>[2x]MAHHHHHHEAVVTPWSVEGDVNYDKLIKDFGSHAIDEALLERIERVLGKKPHHFLRRGIFFSHRDLNLLLDV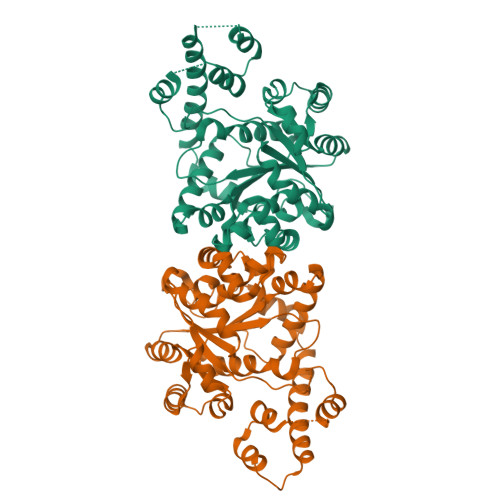YESGQPFYLYTGRGPSSESMHMGHLIPFMFTKWLQDSFRVPLVIQMTDDEKFYFRNIPMEQVEAMTTENIKDIIAMGFDPELTFIFRDFDYMGCMYRTVAKIERAFTASQVRGCFGFAMEDNCGRWMFPAIQAAPSFSAAFPHIFPPSMGNVFCLIPQAIDQDPYFRLTRDIAPRLGYLKPAVIHSKFFPGLSGPKGKMSSSSGTAVLLTDTEKMVKDKINKHAFSGGGATKQEHFLLGANVEVDVPIQWLSFFLEDDEELARVKKEYMLGRIMTGEVKKLLINTITAITKTHQEKRKLVTDEDVQLFTSTRIMGPAKKAATQ> MNYRIIPVTAFSQNCSLIWCEQTRLAALVDPGGDAEKIKQEVDASGVTLMQILLTHGHLDHVGAASELAQHYGVPVIGPEKEDEFWLQGLPAQS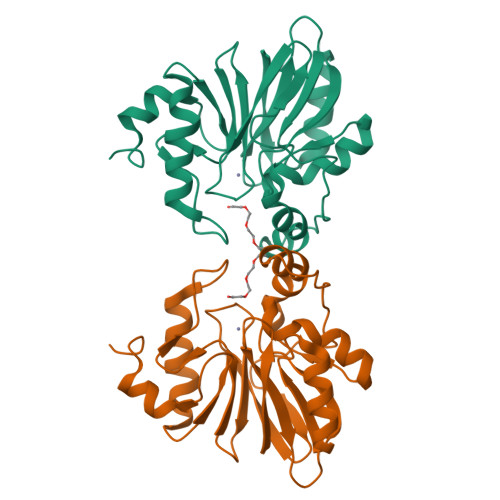RMFGLDECQPLTPDRWLNDGDRVSVGNVTLQVLHCPGHTPGHVVFFDEQSQLLISGDVIFKGGVGRSDFPRGDHTQLIDAIKRKLLPLGDDVTFIPGHGPLSTLGYERLHNPFLQD> SWQTYVDEHLMCDIDGQGQQLAASAIVGHDGSVWAQSSSFPQFKPQEITGIMKDFEEP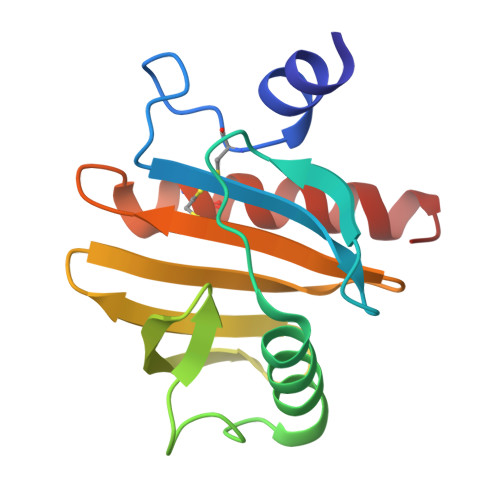GHLAPTGLHLGGIKYMVIQGEAGAVIRGKKGSGGITIKKTGQALVFGIYEEPVTPGQCNMVVERLGDYLIDQGL>[2x]GSIMRDINKLEEQNPDIVSEKKPATEVDPTHFEKRFLKRI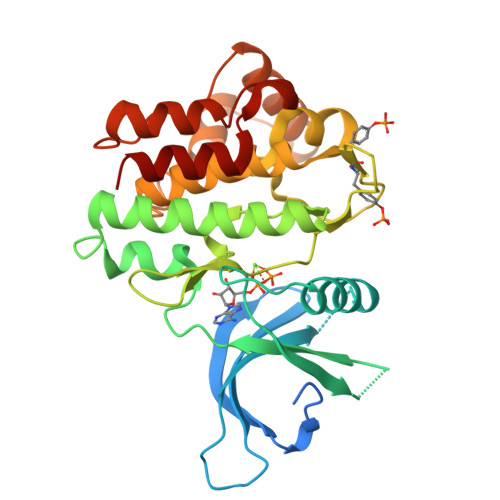RDLGEGHFGKVELCRYDPEGDNTGEQVAVKSLKPESGGNHIADLKKEIEILRNLYHENIVKYKGICTEDGGNGIKLIMEFLPSGSLKEYLPKNKNKINLKQQLKYAVQICKGMDYLGSRQYVHRDLAARNVLVESEHQVKIGDFGLTKAIETDKEYYTVKDDRDSPVFWYAPECLMQSKFYIASDVWSFGVTLHELLTYCDSDSSPMALFLKMIGPTHGQMTVTRLVNTLKEGKRLPCPPNCPDEVYQLMRKCWEFQPSNRTSFQNLIEGFEALLK> MLAGVKKDIEKLYEAVPQLSNVFKIEDKIGEGTFSSVYLATAQLQVGPEEKIALKHLIPTSHPIRIAAELQCLTVAGGQDNVMGVKYCFRKNDHVVIAMPYLEHESFLDILNSLSFQEVREYMLNLFKALKRIHQFGIVHRDVKPSNFL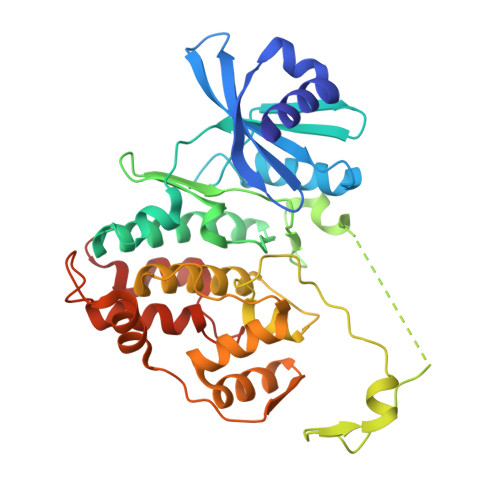YNRRLKKYALVDFGLAQGTHDTKIELLKFVQSEAQQERCSQNKPASLTCDCYATDKVCSICLSRRQQVAPRAGTPGFRAPEVLTKCPNQTTAIDMWSAGVIFLSLLSGRYPFYKASDDLTALAQIMTIRGSRETIQAAKTFGKSILCSKEVPAQDLRKLCERLRGAGAGGWNEVPDEAYDLLDKLLDLNPASRITAEEALLHPFFKDMSL(3E,5E)-6,10-dimethylundeca-3,5,9-trien-2-one | 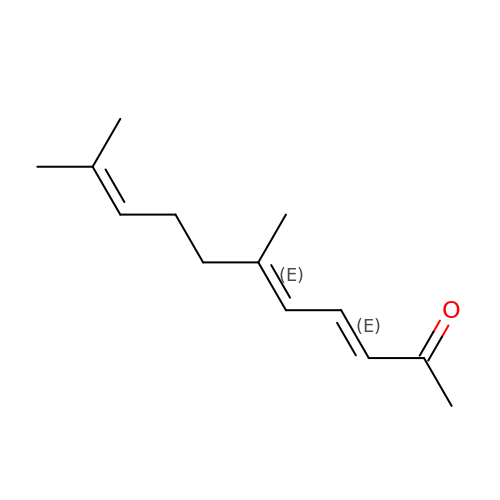C13 H20 O | JXJIQCXXJGRKRJ-KOOBJXAQSA-N> SPDKKWLGTPIEEMRRMPRCGIRLPLLRPSANHTVTIRVDLLRAGEVPKPFPTHYKDLWDNKHVKMPCSEQNLYPVEDENGERTAGSRWELIQTALLNKFTRPQNLKDAILKYNVAYSKKWDFTALIDFWDKVLEEAEAQHLYQSILPDMVKIALCLPNICTQPIPLLKQKMNHSITMSQEQIASLLANAFFCTFPRRNAKMKSEYSSYPDINFNRLFEGRSSRKPEKLKTLFCYFRRVTEKKPTGLVTFTRQSLEDFPEWERCEKPLTRLHVTYEGTIEE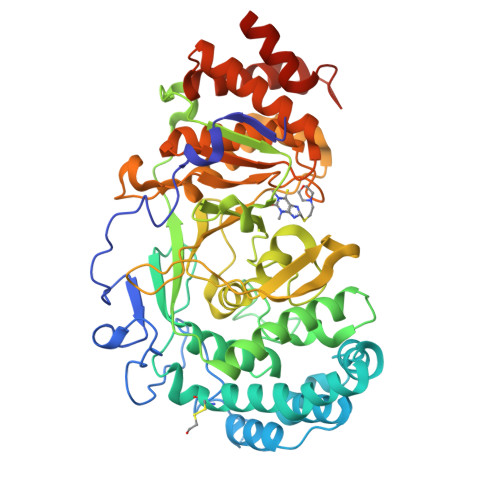NGQGMLQVDFANRFVGGGVTSAGLVQEEIRFLINPELIISRLFTEVLDHNECLIITGTEQYSEYTGYAETYRWSRSHEDGSERDDWQRRCTEIVAIDALHFRRYLDQFVPEKMRRELNKAYCGFLRPGVSSENLSAVATGNWGCGAFGGDARLKALIQILAAAAAERDVVYFTFGDSELMRDIYSMHIFLTERKLTVGDVYKLLLRYYNEECRNCSTPGPDIKLYPFIYHAVESCAETADHSGQRTGT>MVEIIPVSTTLELRAADESHVPALHQLVLKNKAWLQQSLDWPQYVTSQEETRKHVQGNILLHQRGYAKMYLIFCQNEMAGVLSFNAIEPINKAAYIGYWLDESFQGQGIMSQSLQALMTHYARRGDIRR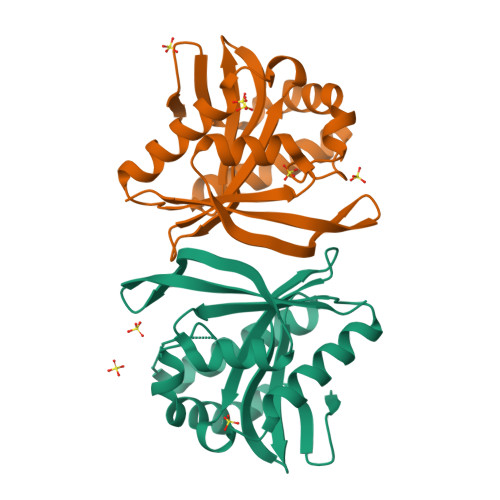FVIKCRVDNQASNAVARRNHFTLEGCMKQAEYLNGDYHDVNMYARIIDAD[2x]> MPEQAVTLEALYAAIEQVLRERLPEAQLIGFWPGVPENTPAVSLEIAELLPERDPGTGESALLCRLQARIMVPPGADRQAVSIACGI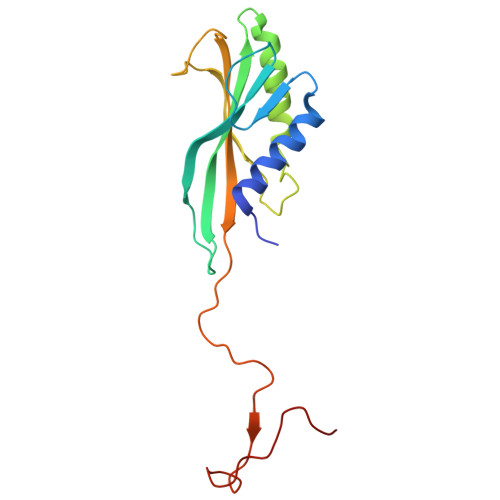VRTLREQTWNLSLQPARFVRSAVDGSREELKSLRVWLVEWTQSLRLGDPEWAWEDQPPGSLMLGFDPQTGPGHEPDYFAPEALA> MLVSVYLALLVACVGQAHSQANLMRLKSDLFNRSPMYPGPTKDDPLTVTLGFTLQDIVKVDSSTNEVDLVYYEQQRWKLNSLMWDPNEYGNITDFRTSAADIWTPDITAYSSTRPVQVLSPQIAVVTHDGSVMFIPAQRLSFMCD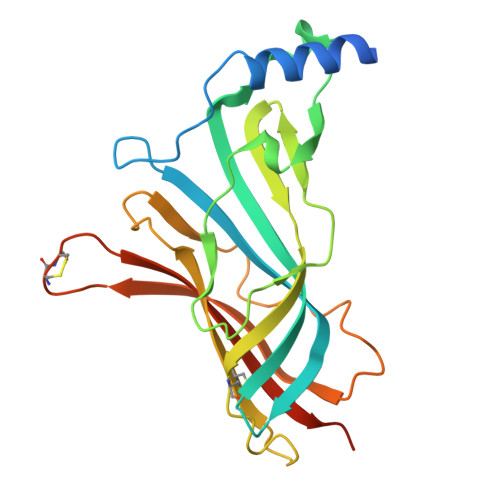PTGVDSEEGVTCAVKFGSWVYSGFEIDLKTDTDQVDLSSYYASSKYEILSATQTRQVQHYSCCPEPYIDVNLVVKFRERRAGNGFFRNLFD>GAAAMRRSEVLAEESIVCLQKALNHLREIWELIGIPEDQRLQRTEVVKKHIKELLDMMIAEEESLKERLIKSISVCQKELNTLCSELHVEPFQEEGETTILQLEKDLRTQVELMRKQKKERKQELKLLQEQDQELCEILCMPHYDIDSASVPSLEELNQFRQHVTTLRETKASRREEFVSIKRQIILCMEELDHTPDTSFERDVVCEDEDAFCLSLENIATLQKLLRQLEMQKSQNEAVCEGLRTQIRELWDRLQIPEEEREAVATIMSGSKAKVRKALQLEVDRLEELKMQNMKKVIEAIRVELVQYWDQCFYSQEQRQAFAPFCAEDYTESLLQLHDAEIVRLKNYYEVHKELFEGVQKWEETWRL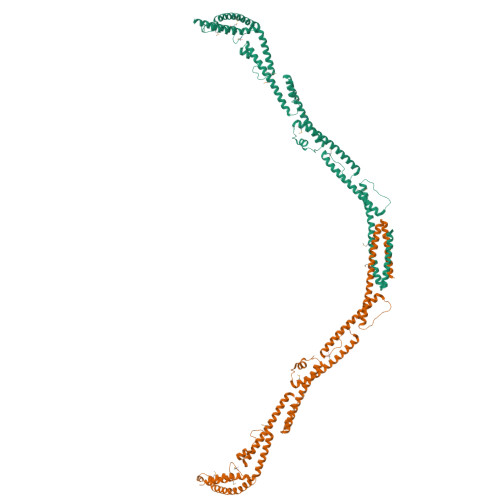FLEFERKASDPNRFTNRGGNLLKEEKQRAKLQKMLPKLEEELKARIELWEQEHSKAFMVNGQKFMEYVAEQWEMHRLEKERAKQERQLKNKKQTETEMLYGSAPRTPSKRRGLAPNTPGKAR[2x]> GMYANKVKKIAAVHDLSGMGRVSLTVVIPILSSMGFQVCPLPT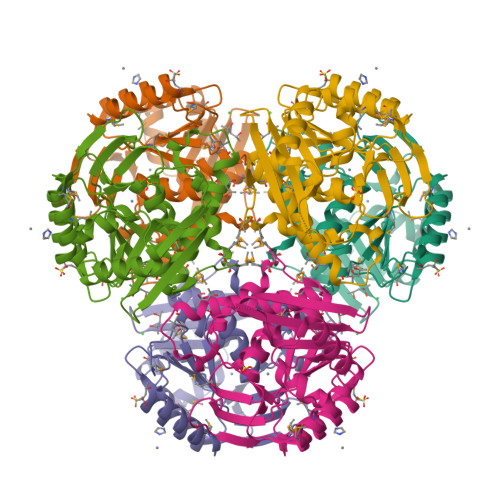AVLSNHTQYPGFSFLDLTDEMPKIIAEWKKLEVQFDAIYTGYLGSPRQIQIVSDFIKDFRQPDSLIVADPVLGDNGRLYTNFDMEMVKEMRHLITKADVITPNLTELFYLLDEPYKADSTDEELKEYLRLLSDKGPQVVIITSVPVHDEPHKTSVYAYNRQGNRYWKVTCPYLPAHYPGTGDTFTSVITGSLMQGDSLPMALDRATQFILQGIRATFGYEYDNREGILLEKVLHNLDMPIQMASYELI> GLKQKIVIKVAMEGNNCRSKAMALVASTGGVDSVALVGDLRDKIEVVGYGIDPIKLISALRKKVGDAELLQVSQA;> GPAPARFCVYYDGHLPATRVLLMYVRIGTTATITARGHEFEVEAKDQNCKVILTNGKQA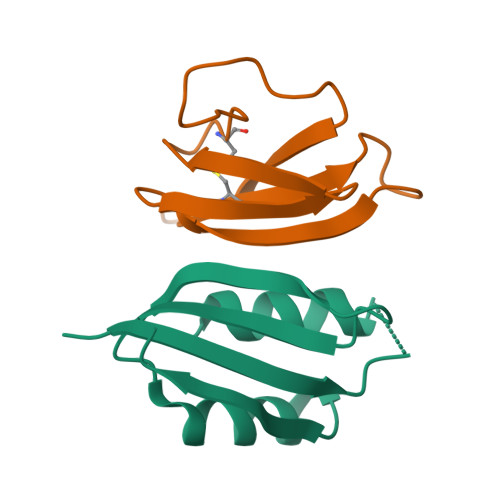PDWLAAEPY> AAPGKPTIAWGNTKFAIVEVDQAATAYNNLVKVKNAADVSVSWNLWNGDTGTTAKVLLNGKEAWSGPSTGSSGTANFKVNKGGRYQMQVALCNADGCTASDATEIVVADTDGSHLAPLKEPLLEKNKPYKQNSGKVVGSYFVEWGVYGRNFTVDKIPAQNLTHLLYGFIPICGGNGINDSLKEIEGSFQALQRSCQGREDFKVSIHDPFAALQKAQKGVTAWDDPYKGNFGQLMALKQAHPDLKILPSIGGWTLSDPFFFMGDKVKRDRFVGSVKEFLQTWKFFDGVDIDWEFPGGKGANPNLGSPQDGETYVLLMKELRA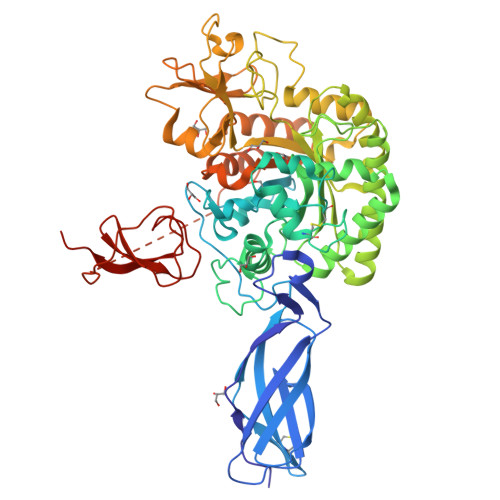MLDQLSVETGRKYELTSAISAGKDKIDKFYSFVNVAQNSMDHIFLMSYDFYGAFDLKNLGHQTALNAPAWKPDTAYTTVNGVNALLAQGVKPGKIVVGTAMYGRGWTGVNGYQNNIPFTGTATGPVKGTWENGIVDYRQIAGQFMSGEWQYTYDATAEAPYVFKPSTGDLITFDDARSVQAKGKYVLDKQLGGLFSWEIDADNGDILNSMNASLGAADYDDSQLDMGTGLRYTGVGPGNLPIMTAPAYVPGTTYAQGALVSYQGYVWQTKWGYITSAPGSDSAWLKVGRVAHHHHHH>MVSAGIEAMNVFGGTAYLDVMELAKYRHLDTARFENLLM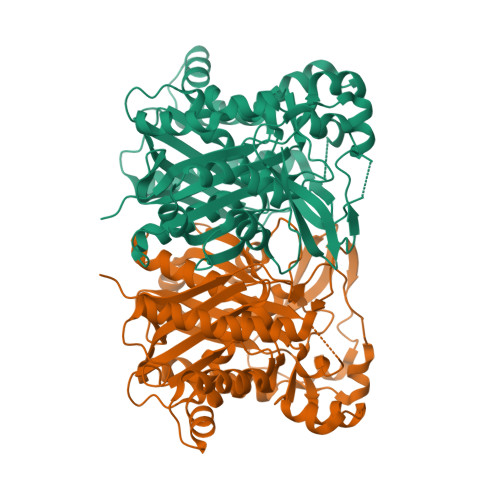KEKAVALPYEDPVTFGVNAAKPIIDALSEAEKDRIELLITCSASGIDFGKSLSTYIHEYLGLNRNCRLFEVKQACYSGTAGFQMAVNFILSQTSPGAKALVIASDISRFLIAEGGDALSEDWSYAEPSAGAGAVAVLVGENPEVFQIDPGANGYYGYEVMDTCRPIPDSEAGDSDLSLMSYLDCCEQTFLEYQKRVPGANYQDTFQYLAYHTPFGGMVKGAHRTMMRKVAKVKTSGIETDFLTRVKPGLNYCQRVGNIMGAALFLALASTIDQGRFDTPKRIGCFSYGSGCCSEFYSGITTPQGQERQRTFGIEKHLDRRYQLSMEEYELLFKGSGMVRFGTRNVKLDFEMIPGIMQSTQEKPRLFLEEISEFHRKYRWIS[2x]>GSMALEQALQAARRGDLDVLRSLHAAGLLGPSLRDSLDALPVHHAARSGKLHCLRYLVEEVALPAVSRARNGATPAHDAAATGYLSCLQWLLTQGGCRVQEKDNSGATVLHLAARFGHPDVVKWLLYQGGANSAITTDTGALPIHYAAAKGDLPSLKLLVGHYPEGVNAQTNNGATPLYLACQEGHLEVTKYLVQECSADPHLRAQDGMTPLHAAAQMGHNPVLVWLVSFADVSFSEQDHDGATAMHFAASRGHTKVLSWLLLHGAEISQDLWGGTPLHDA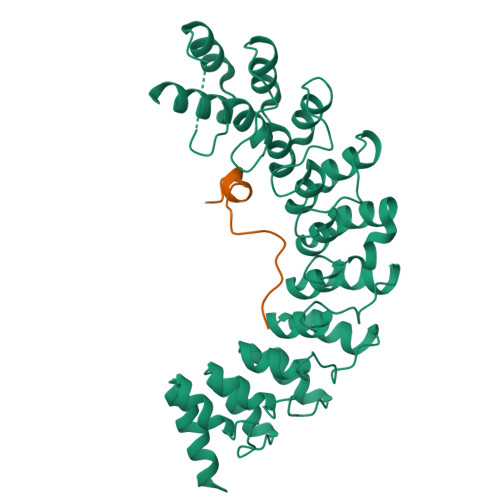AENGELECCQILAVNGAGLDVRDHDGYTAADLAEFNGHTHCSRYLRTVQTLSLEHRVLSRDQSMDLEAKQLDS[2x];>SQRKPRKLGQIKVLDGEDQYYKCLSPGACAPEETHSVHPFFFSSSPREDPFAQH[2x]> VYLDRKLLTLEDKELGSGNFGTVKKGYYQMKKVVKTVAVKILKNE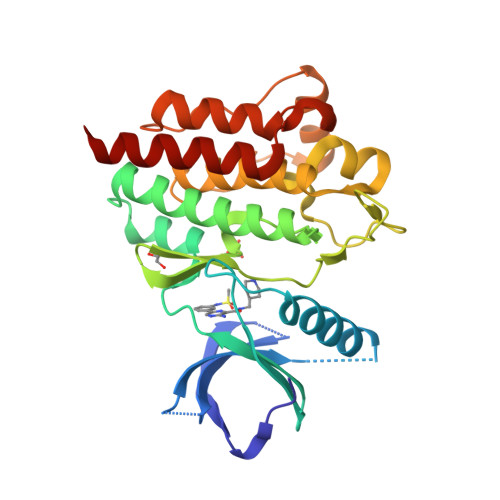ANDPALKDELLAEANVMQQLDNPYIVRMIGICEAESWMLVMEMAELGPLNKYLQQNRHVKDKNIIELVHQVSMGMKYLEESNFVHRDLAARNVLLVTQHYAKISDFGLSKALRADENYYKAQTHGKWPVKWYAPECINYYKFSSKSDVWSFGVLMWEAFSYGQKPYRGMKGSEVTAMLEKGERMGCPAGCPREMYDLMNLCWTYDVENRPGFAAVELRLRNYYYDVVNE>MTMYVIKRSGRKEKLDINKIRIAIKFACEGLNVDPLELEADAQIQFRDGITTKEIQQLLIKTAAEKVSAERPDWTYTAARLLLYDLYKDVAHLRGYSLRDDLGKYKPYNRKNFYSFVKEYVEKGIYGEYLLENYSEEDFNKLANYIKPERDLYFTYTGIKILYDRYLVRDEEGRVIELPQEMYMLIAMTLAVPEKPEERLKWAKKFYDVLSEHKVTVATPTLMNARRPFTQLSSC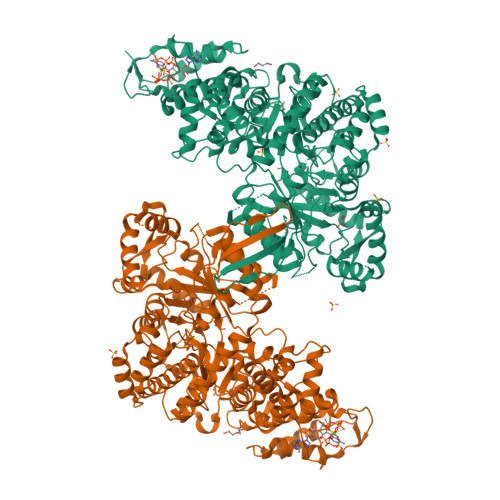FVLTVDDDLFDIFDNVKKAGMISKFAGGLGVYLGKIRATGAPIRKFKGASSGVIPVVKLINDTMTYVDQLGMRKGSASITLDIWHKDILDFLEVKTNVGDERKKAHDIHPAVSIPDLFMKRLKNREDWTLIDPYWARQYITRKIYDGKYKEVKPLPGSHYYVGIKEDGTQDILEPKGLEDFYGEEFEKWYLELEENLPSYAKKKVNSFELWKRLLTVAFETGEPYIFFRDEANRKNPNKHTGMVYSSNLCHEIVQTMSPSKHEKPVLDPETGEITYKKEAGDLPVCNLGSVNLGKVHTEEEIKEVLPLLVRMLDNVIEMNFYAIPEAEYTNKRYRAIGIGVSNYHYCLVKNGIKWESEEHLKFADKLFELIAFYALKGSLELAKERGRYKLFDGSNWSKGILFGRSVEEIEENSRQNGNNLPWRELAEEIKKYGIRNAYLLALMPTGSTSLILGATPSIDPIFARFYKEENMSGILPQVPPEVDRFYWHYKTAYTIDHEWTIRAAAVRQKWIDQAQSLNLFVDPQNIDGPRLSRLYELAWELGLKTIYYLRSRSAMDIEECEACSV[2x]> HMHFTIQREALLKPLQLVAGVVERRQTLPVLSNVLLVVEGQQLSLTGT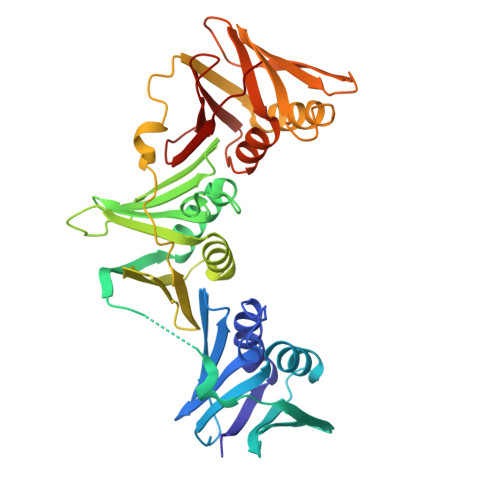DLEVELVGRVVLEDAAEPGEITVPARKLMDICKSLPNDVLIDIRVEEQKLLVKAGRSRFTLSTLPANDFPTVEEGPGSLNFSIAQSKLRRLIDRTSFAMAQQDVRYYLNGMLLEVNGGTLRSVATDGHRLAMCSLDAQIPSQDRHQVIVPRKGILELARLLTEQDGEVGIVLGQHHIRATTGEFTFTSKLVDGKFPDYERVLPRGGDKLVVGDRQQLREAFSRTAILSNEKYRGIRLQLSNGLLKIQANNPEQEEAEEEVQVEYNGGNLEIGFNVSYLLDVLGVIGTEQVRFILSDSNSSALVHEADNDDSAYVVMPMRL> GSTGSPPGPPTSIHVEEITDTTATLSWRPGPDNHSPITAYTIQARTPFSLGWQAVSTVPEVVGGSHLTATVIELNPWVEYEFRVLASNAVGTGEPSKPSKKARTKDTVPKVTPANVSGGGGSRSELVITWEPVPEELQNGAGFGYVVAFRPFGSTGWMQAAVPSPEASKYVFKNETILPFSPFQVKVGAYNNKGEGPFGPVITIYSAEEEPGRAPSRLRAKSLSASDVEVSWKALPWSTSKKRVLGYELRYWEKNEKEDASSVLRTVGNRTLAIIQGLKGSSTYYITVRAYNTAGTGPPSPVVNITTKK;> GPGSIEVPSDDSVGLLAEPQVAMFCGKLNMHINVQSGKWEPDPTGTKSCISTKEGILKYCQEVYPDLQITNVVEANQPVSIQNWCKMGRRQCRSHTHIVVPYRCLVGEFVSDALLVPDKCKFLHQERMDMCESHLHWHTVAKESCGDRSMNLHDYGMLLPCGIDRFRGVEFVCCPMEEQKDLDSEAAA

Contactins (CNTNs) are neural cell adhesion molecules that encode axon-target specificity during the patterning of the vertebrate visual and olfactory systems. Because CNTNs are tethered to the plasma membrane by a glycosylphosphatidylinositol anchor, they lack an intracellular region to communicate across the membrane. Instead, they form coreceptor complexes with distinct transmembrane proteins to transmit signals inside the cell. Finally, structural analyses of five CNTN–amyloid pairs indicate that these proteins interact through a conserved interface involving the second fibronectin type III repeat of CNTNs and the copper-binding domain of amyloid proteins.

Human APP appears more closely related to APPb than APPa, so we crystallized the E1 domain of APPb and the FN1–FN3 region of zebrafish CNTN4. Surprisingly, subsequent structural analysis indicated that a proteolytic event had likely released the growth factor–like domain of APPb so that only its copper-binding domain bound to CNTN4 (2.93 Å, Rwork/Rfree = 0.241/0.281). Overall, the CNTN4–APPb and CNTN4–APLP2 interfaces display many of the same features found in the cocrystals of chicken CNTN4 and APP. As is the case in previous CNTN–APP complex structures, the bulk of the interactions includes main chain–main chain hydrogen bonds between two β-strands: W751–Q753 in CNTN4 and L129–P132 in APPb or L134–P137 in APLP2. As is the case in the CNTN3–APP and CNTN4–APP interfaces, the carbonyl oxygen atom of S126 in APPb (S131 in APLP2) forms a hydrogen bond with the hydroxyl group of Y764. Furthermore, CNTN4 residues Y784 and E789 form hydrogen bonds with E141 and H139, respectively, in APPb, and with E146 and H144, respectively, in APLP2. These contacts are absent in the chicken CNTN4–APP and mouse CNTN5–APP complexes. Overall, the sum of this crystallographic work indicates that the CNTN4–APLP2 interface in zebrafish is essentially identical to the CNTN4–APPb interface in zebrafish and the CNTN4–APP interface in chicken.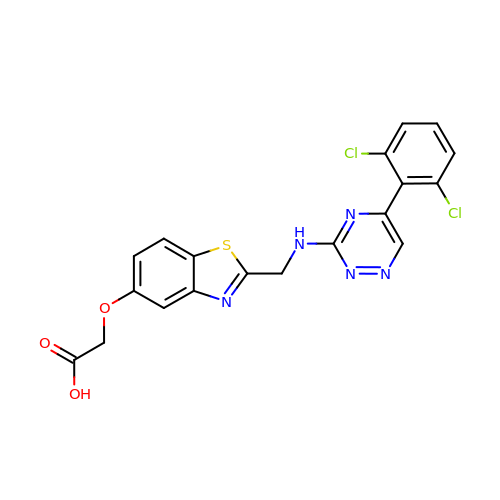{[2-({[5-(2,6-dichlorophenyl)-1,2,4-triazin-3-yl]amino}methyl)-1,3-benzothiazol-5-yl]oxy}acetic acid | C19 H13 Cl2 N5 O3 S | VNZNZAJGDVEIIU-UHFFFAOYSA-N> MSTLCPPPSPAVAKTEIALSGKSPLLAATFAYWDNILGPRVRHIWAPKTEQVLLSDGEITFLANHTLNGEILRNAESGAIDVKFFVLSEKGV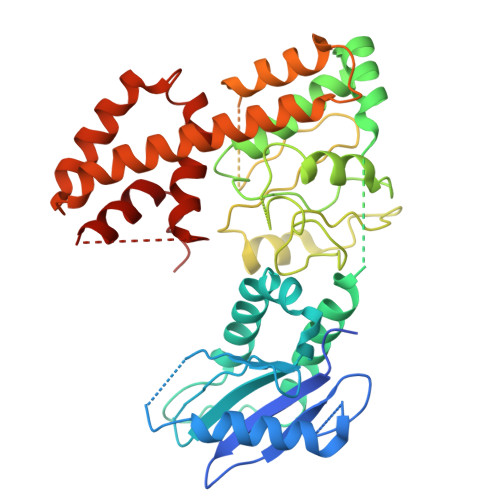IIVSLIFDGNWNGDRSTYGLSIILPQTELSFYLPLHRVCVDRLTHIIRKGRIWMHKERQENVQKIILEGTERMEDQGQSIIPMLTGEVIPVMELLSSMKSHSVPEEIDIADTVLNDDDIGDSCHEGFLLNAISSHLQTCGCSVVVGSSAEKVNKIVRTLCLFLTPAERKCSRLCEAESSFKYESGLFVQGLLKDSTGSFVLPFRQVMYAPYPTTHIDVDVNTVKQMPPCHEHIYNQRRYMRSELTAFWRATSEEDMAQDTIIYTDESFTPDLNIFQDVLHRDTLVKAFLDQVFQLKPGLSLRSTFLAQFLLVLHRKALTLIKYIEDDTQKGKKPFKSLRNLKIDLDLTAEGDLNIIMALAEKIKPGLHSFIFGRPFYTSVQERDVLMTF> GSPISPIETVPVKLKPGMDGPKVKQWPLTEEKIKALVEICTEMEKEGKISKIGPENP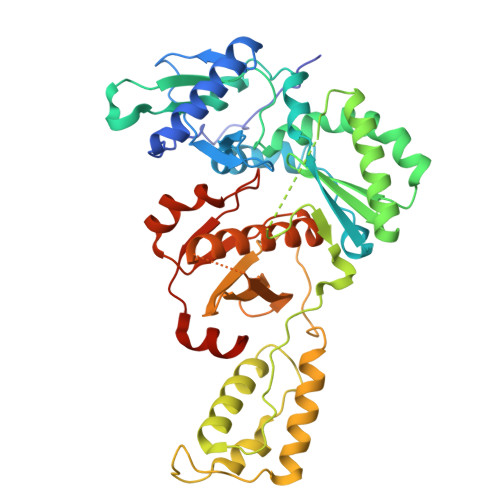YNTPVFAIKKKDSTKWRKLVDFRELNKRTQDFWEVQLGIPHPAGLKKKKSVTVLDVGDAYFSVPLDEDFRKYTAFTIPSINNETPGIRYQYNVLPQGWKGSPAIFQSSMTKILEPFRKQNPDIVIYQYMDDLYVGSDLEIGQHRTKIEELRQHLLRWGLTTPDKKHQKEPPFLWMGYELHPDKWTVQPIVLPEKDSWTVNDIQKLVGKLNWASQIYPGIKVRQLCKLLRGTKALTEVIPLTEEAELELAENREILKEPVHGVYYDPSKDLIAEIQKQGQGQWTYQIYQEPFKNLKTGKYARMRGAHTNDVKQLTEAVQKITTESIVIWGKTPKFKLPIQKETWETWWTEYWQATWIPEWEFVNTPPLVKLWYQLEKEPIVGAETF> MSTFSGDETAP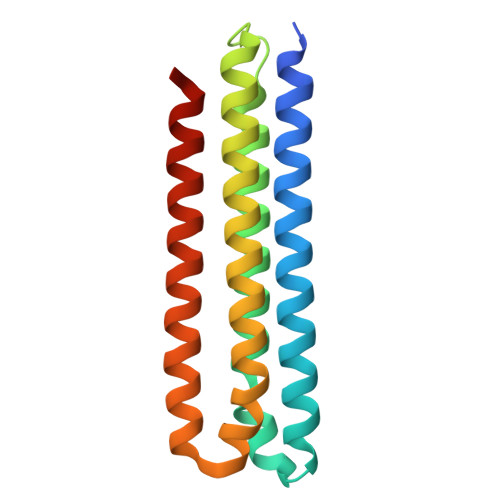FFGFLGAAAALVFSCMGAAYGTAKSGVGVASMGVMRPELVMKSIVPVVMAGVLGIYGLIIAVIISTGINPKAKSYYLFDGYAHLSSGLACGLAGLSAGMAIGIVGDAGVRANAQQPKLFVGMILILIFAEALALYGLIVGIILSSRAGQSRAE>[2x]MIKQIGRFFRAFIFIMPLSLTSCESKIDRNRIWIVGTNATYPPFEYVDAQGEVVGFDIDLAKAISEKLGKQLEVREFAFDALI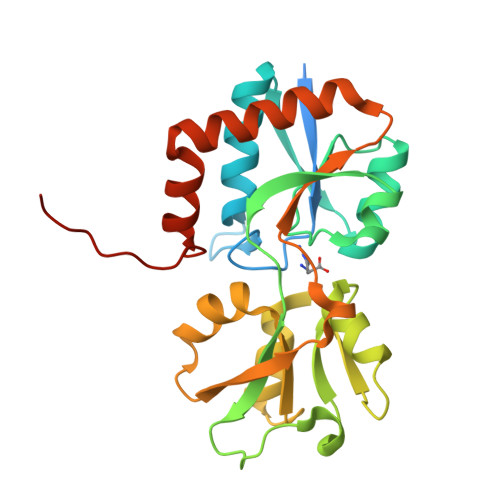LNLKKHRIDAILAGMSITPSRQKEIALLPYYGDEVQELMVVSKRSLETPVLPLTQYSSVAVQTGTYQEHYLLSQPGICVRSFDSTLEVIMEVRYGKSPVAVLEPSVGRVVLKDFPNLVATRLELPPECWVLGCGLGVAKDRPEEIQTIQQAITDLKSEGVIQSLTKKWQLSEVAYEAAQVWGHTP> APSVKGVSFDQANNLLIEPARIEEEELTLTILRQTGGLGISIAGGKGSTPYKGDDEGIFISRVSEEGPAARAGVRVGDKLLEVNGVALQGAEHHEAVEALRGAGTAVQMRVWRERM;> 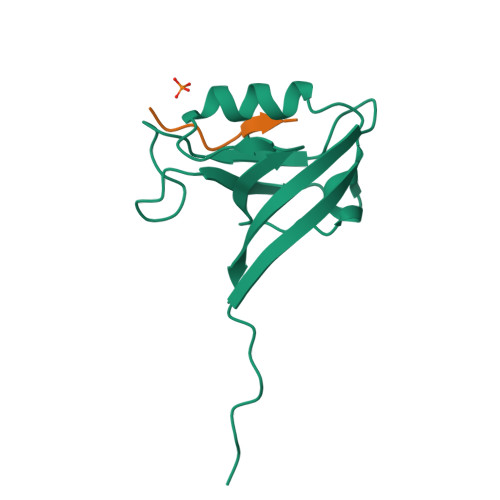QEEWETVM>MAHHHHHHMSLVEVLPNYFTLSKDSPLRKKFEKVYKWYSPAFSPHDVPRFAEVGNITENPEVMRGIRDFFVDRYKNLQQPITHILGFDSRGFLLGPMIAVELNVPFVLIRKANKIAGVIIKSEPYTKEYAAESEECMTVRFGSFDKNSRVVLIDDVIATGGTMLAGVQLVDACGATLVEVAGILGLTFLKGTQPAHTFAGGRYSNVPFVTLVDETVLSDENCGDPL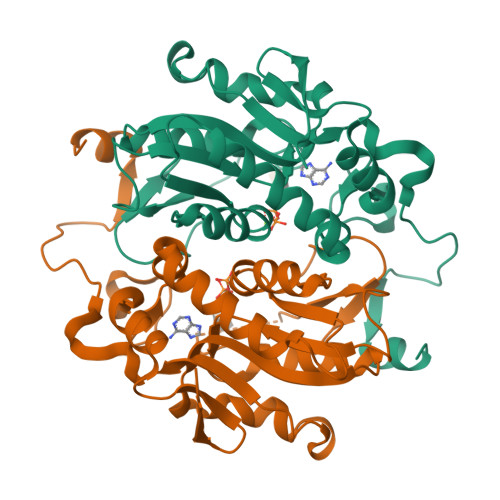HHKGSRIISCAEAKKLI[2x]2-[(3,5-difluoro-4-hydroxyphenyl)amino]-8-phenyl-7,8-dihydropteridin-6(5H)-one | C18 H13 F2 N5 O2 | 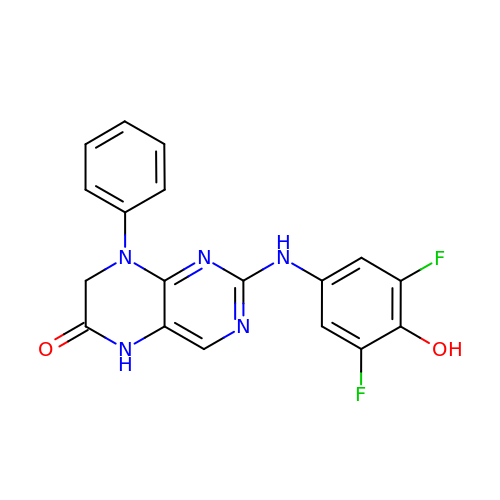LGIWSHCSALMSPR-UHFFFAOYSA-N> GAMGSHMEFMDYDFKVKLSSERERVEDLFEYEGCKVGRGTYGHVYKAKRKDGKDDKDYALKQIEGTGISMSACREIALLRELKHPNVISLQKVFLSHADRKVWLLFDYAEHDLWHIIKFHRASKANKKPVQLPRGMVKSLLYQILDGIHYLHANWVLHRDLKPANILVMGEGPERGRVKIADMGFARLFNSPLKPLADLDPVVVTFWYRAPELLLGARHYTKAIDIWAIGCIFAELLTSEPIFHCRQEDIKTSNPYHHDQLDRIFNVMGFPADKDWEDIKKMPEHSTLMKDFRRNTYTNCSLIKYMEKHKVK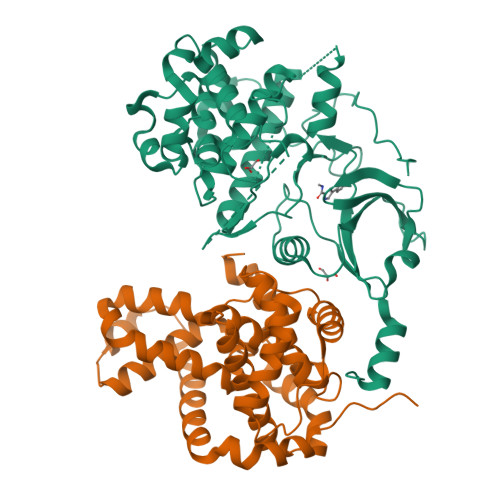PDSKAFHLLQKLLTMDPIKRITSEQAMQDPYFLEDPLPTSDVFAGCQIPYPKREFLTEEEPDDKGDKK;> AGNFWQSSHYLQWILDKQDLLKERQKDLKFLSEEEYWKLQIFFTNVIQALGEHLKLRQQVIATATVYFKRFYARYSLKSIDPVLMAPTCVFLASKVEEFGVVSNTRLIAAATSVLKTRFSYAFPKEFPYRMNHILECEFYLLELMDCCLIVYHPYRPLLQYVQDMGQEDMLLPLAWRIVNDTYRTDLCLLYPPFMIALACLHVACVVQQKDARQWFAELSVDMEKILEIIRVILKLYEQWKNFDERKEMATILSKMPKPKPPP> SNADTIKVGVIGTMSGPYALFGKNYKMGIDAWVAEHGNKVAGHTVEFVYRDEVSPNPAQSKALAQELIVKEKVQYLAGLYFTPNAMAVAPLLQEAKVPMVVMNAATSSITEKSPYIVRTSFTMFQNTVPAAKVAKQKGATKVAIAVSDYGPGIDAETAFKKTFEAEGGKVVEAVRMPLSTTDFGPIMQRIKNSGADMIFTFLPAGPPTLGFVKAYIDNGLKAGGVKLMSTGDVVTEPDLPNIGEAGLGILSTYHYAVSHDSPENKAFLALLQKGGAKLDEVTMTSVAAYDGARLIYKMIEATSGKSDPDKAIAAVKGMKWVSPRGEVSIDPETRHITQNVYLREVEKVDGKLINRELETF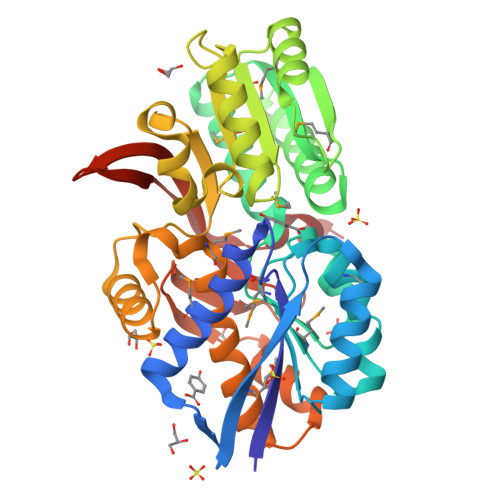KAQPDWGLAKQ> MEDINFASLAPRHGSRPFMGNWQDIGTSNMS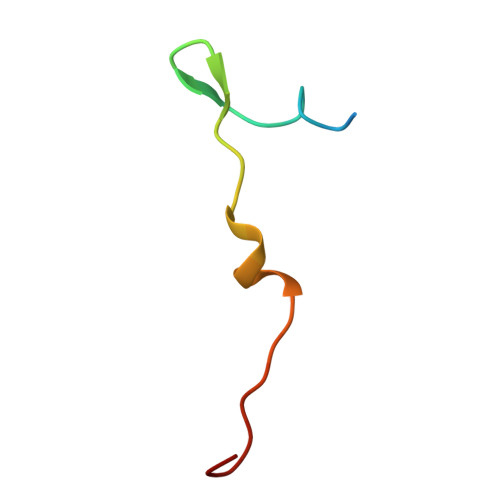GG C-(1-AZIDO-ALPHA-D-GLUCOPYRANOSYL) 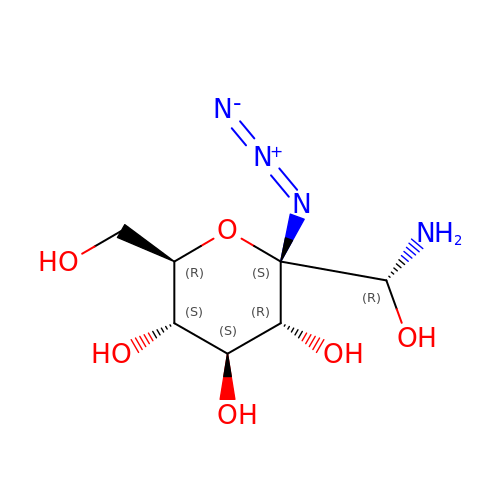FORMAMIDE | C7 H14 N4 O6 | LAKOUYZWWLMCSL-JBFGQTLDSA-N>GMAEPNGQSAPNGTTSNGRPSYAEKHKLPAHFIGGNRLENAPPSKVKDFVAEHGGHTVITNVLIANNGIAAVKEIRSVRKWAYETFGDERAIKFTVMATPEDLQANADYIRMADHYVEVPGGTNNHNYANVELIVDVAERMDVHAVWAGWGHASENPKLPESLAASPKKIVFIGPPGSAMRSLGDKISSTIVAQHANVPTIPWSGSGVSEVHIDENGIVTVPEEVYLKGCVNSWEEGLEKAREIGFPVMIKASEGGGGKGIRKCMNEDQFEELYKAAAAEIPGSPIFIMKLADSARHLEVQLLADQYGNNISLFGRDCSVQRRHQKIIEEAPVTIASPTTFRAMEEAAVRLGKLVGYVSAGTVEYLYSHADDKFYFLELNPRLQVEHPTTEMVSGVNLPAAQLQIAMGIPLHRIRDIRLLYGVDPKAATEIDFEFKNPESEKTQRRPAPKGHTTACRITSEDPGEGFKPSSGMLQELNFRSSSNVWGYFSVGTAGGIHSFSDSQFGHIFAYGENRAASRKHMIVALKELSIRGDFRTTVEYLIKLLETQAFEENTITTGWLDELISKKLTAERPDTNLAIICGAVIRAHTESEKSLADYRAGLEKGQVPSKDILKTVSSVDFIYEGLRYKFTVTRSSVDTYRLFINGSQCEVGVRTLSDGGLLVLLGGHSHNVYWKDEATGTRISIDGKTCLLEQENDPTGSGALDDPSRVKQAQPFVGQLPQYGSPVVVGSKPAQRFAVLYGTMCDILNGYDNQVVMQQKLKEFIEVLRDPKLPYSEFSAQFSALHARMPHKLDAQLTQVLERAQNRGAEFPARQLLKVFNKFLDDNVPNKTDQDLLKSTLEPLTSVLNLYLDGQKARELNLIADLLSMYADVECQFSGRRLQDEEAILKLRDQYKDNIQKVVNTVLSHKNVMSKNSLVLALLDEYRPNKPNVGNVGKHLRPVLRRLTELESRQSAKVSLKAREVLILCALPSLEERTAQMEHILRSSVVQSRYGETGWSHRRPDREVLKEVVDSKYTVFDVLTLFFAHEDPYVALAALEVYVRRAYRAYNLREVRYHDEERPYFIDWDFALRKSGANQTESSMHMQSVVPSSPATPVENDFKRIHSISDMTYLARRTRDEPIRKGVIVPCKDLLDAEEALSRALEVLPLAHKETKDKDRKQQPGIAADLAQRRRPGTPLRLEGIGELSAVVNVAVRDAEGKNDEEILALIKPWVQNSKADLLARRVRRLTFICGRNDGSYPSYYTFRGPDYAEDDSIRHIEPSLAFQLELGRLSKFKLTPVFTQNKNIHVYEAVGRGVETDRRYFTRAVVRPGRLRDEISTAEYLISEADRVVNDIFDALEIIGTNKTDLNHMFINFSHTFQVTADEVAESLQGFLDRFGPRGWRLRVHQVEIRINCMRSDNNDENDTMPLRVIITNTSGFVIQIELYEEKLSEKGEWVYYYVSGNAKIGSMHLLPVSTPYPTKNWLQPKRYKAHILGTQYVYDFPELFRQAIQNSWTEAVKKIPSLAAKQPAIGECIDYNELVLGDQDNLAEVSREPGMNSTGMVGWLINARTPEYPDGRKFIVVANDITFKIGSFGPKEDTFFFKCTELARKMGIPRIYLSANSGARLGLAEELMPHFNVAWNDPAKPEAGFKYLYLSDEAKRRFENEVITEEIVEDGEKRHKIITIVGAEEGLGVECLRGSGLIAGATSRAYNDIFTCTLVTCRSVGIGAYLVRLGQRAVQVEGQPIILTGAPALNSLLGREVYTSNLQLGGTQIMYRNGVSHLTAKDDFDGVTKIVQWLSFIPDQRNNPLPILSPSPDPWDRDVVYTPPYKQTYDVRWMIAGKEDEDGFQPGLFDKDSFVETLGGWARTVVVGRARLGGIPMGVIAVETRTIENITPADPANPDSIEQVTNEAGGVWYPNSAFKTAQAINDFNYGEQLPLMILANWRGFSGGQRDMYNEVLKYGSFIVDALTRFEKPIFIYIPPHGELRGGSWVVVDPTINPASMEMYADEEARGGVLEPEGIIPIKYKKDKQLETMARLDPVYRSLKKEMAKEGLSKEESDNIKKKMQQREELLLPIYHQICVQFADLHDRAGRMKAKGVIRQSLQWRQSRRFFYWRVRRRLIEDDILRRIEEAINPAGKRRHDPENTSLAASPETRSPHLVQLESWVGIPGFKTNDREVVEWYEQNQDRINEKLEKLKKESIADQMRELLRXXXXXXXXXXXX[2x]

Biotin-dependent acetyl-CoA carboxylases (ACCs) are essential enzymes that catalyse the ATP-dependent carboxylation of acetyl-CoA to malonyl-CoA. Eukaryotic ACCs, instead, are multienzymes, which integrate all functional components into a single polypeptide chain of ∼2,300 amino acids2. In addition to the canonical ACC components, eukaryotic ACCs contain two non-catalytic regions, the large central domain (CD) and the BC–CT interaction domain (BT). Here we provide the structure of Saccharomyces cerevisiae (Sce) ACC CD, intermediate- and low-resolution structures of human (Hsa) ACC CD and larger fragments of fungal ACC from Chaetomium thermophilum (Cth).

To improve crystallizability, we generated ΔBCCP variants of full-length ACC, which, based on SAXS analysis, preserve properties of intact ACC. For CthΔBCCP, crystals diffracting to 8.4 Å resolution were obtained. However, molecular replacement did not reveal a unique positioning of the BC domain. Owing to the limited resolution the discussion of structures of CthCD-CT and CthΔBCCP is restricted to the analysis of domain localization. However, MS analysis of CthCD-CT and CthΔBCCP constructs revealed between 60 and 70% phosphorylation of Ser1170 (corresponding to SceACC Ser1157). The CDN domain positioning relative to CDL/CDC1 is highly variable with three main orientations observed in the structures of SceCD and the larger CthACC fragments: CDN tilts, resulting in a displacement of its N terminus by 23 Å (observed in both protomers of CthCD-CT and one protomer of CthΔBCCP, denoted as CthCD-CT1/2 and CthΔBCCP1, respectively). In addition, CDN can rotate around hinges in the connection between CDN/CDL by 70° (observed in the second protomer of CthΔBCCP, denoted as CthΔBCCP2) and 160° (observed in SceCD) leading to displacement of the anchor site for the BCCP linker by up to 33 and 40 Å, respectively. Conformational variability in the CD thus contributes considerably to variations in the spacing between the BC and CT domains, and may extend to distance variations beyond the mobility range of the flexibly tethered BCCP. Comparison of flACC with our CthΔBCCP structure reveals the CDC2/CT hinge as a major contributor to conformational flexibility.> LEENDC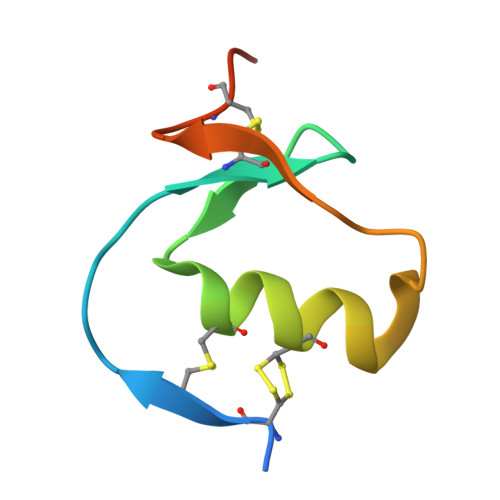ACPRVLHRVCGSDGNTYSNPCTLDCAKHEGKPDLVQVHEGPCDPNDHDF> MSELFGVLKSNAGRIILKDPSATSKDVKAYIDSVINTCKNGSITKKAELDEITVDGLDANQVWWQVKLVLDSIDGDLIQGIQELKDVVTPSHNLSDGSTLNSSSGEESELEEAESVFKEKQMLSADVSEIEEQSNDSLSENDEEPSMDDEKTSAEAAREEFAEEKRISSGQDERHSSPDPYGINDKFFDLEKFNRDTLAAEDSNEASEGSEDEDIDYFQDMPSDDEEEEAIYYEDFFDKPTKEPVKKHSDVKDPKEDEELDEEEHDSAMDKVKLDLFADEEDEPNAEGVGEASDKNLSSFEKQQIEIRKQIEQLENEAVAEKKWSLKGEVKAKDRPEDALLTEELEFDRTAKPVPVITSEVTESLEDMIRRRIQDSNFDDLQRRTLLDITRKSQRPQFELSDVKSSKSLAEIYEDDYTRAEDESALSEELQKAHSEISELYANLVYKLDVLSSVHFVPKPASTSLEIRVETPTISMEDAQPLYMSNASSLAPQEIYNVGKAEKDGEIRLKNGVAMSKEELTREDKNRLRRALKRKRSKANLPNVNK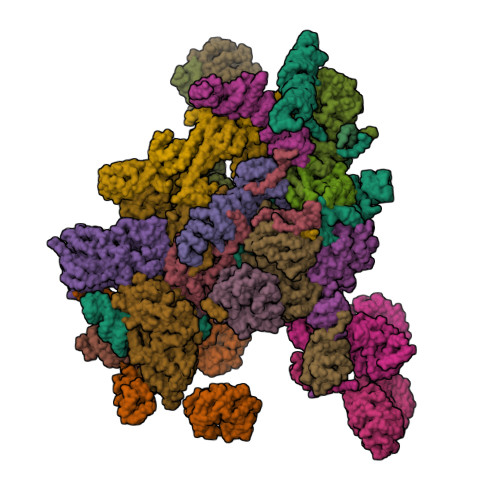RSKRNDVVDTLSKAKNITVINQKGEKKDVSGKTKKSRSGPDSTNIKL;> MSNGHVKFDADESQASASAVTDRQDDVLVISKKDKEVHSSSDEESDDDDAPQEEGLHSGKSEVESQITQREEAIRLEQSQLRSKRRKQNELYAKQKKSVNETEVTDEVIAELPEELLKNIDQKDEGSTQYSSSRHVTFDKLDESDENEEALAKAIKTKKRKTLKNLRKDSVKRGKFRVQLLSTTQDSKTLPPKKESSIIRSKDRWLNRKALNKG;> MTQSLGIEQYKLSVVSGGKPALNNLSSVTGNKNIARLSQDQRNYIIPFNNQIKVYSVETRQCVKTLKFANNSLLSGIFLQEEENNESIVKILLGDITVPQQEDAHLITVFTNNGHVIVLNYKGKLVESPKHFKISLADEKLANVFHSEGNYRILTTFKDPSQKAHNSLQSYRLYALTFDDAKKQFEVAHQAEWHNVILSNISSNGKLLAHMCKDVSTKDHEHKSISVVSLFDDSVNLSFPLGSILSSQTQSLSYNTRYVSSMAIDNMGQQLAVGFASGVISIVSLADLQIRLLKWHIDSVLSLSFSHDGSYLLSGGWEKVMSLWQLETNSQQFLPRLNGIIIDCQVLGPQGNYYSLILQMTENNSNSDYQFLLLNASDLTSKLSINGPLPVFNSTIKHIQQPISAMNTKNSNSITSLNHSKKKQSRKLIKSRRQDFTTNVEINPINKNLYFPHISAVQIFDFYKNEQVNYQYLTSGVNNSMGKVRFELNLQDPIITDLKFTKDGQWMITYEIEYPPNDLLSSKDLTHILKFWTKNDNETNWNLKTKVINPHGISVPITKILPSPRSVNNSQGCLTADNNGGLKFWSFDSHESNWCLKKISLPNFNHFSNSVSLAWSQDGSLIFHGFDDKLQILDFDTFKKFESLENTKTVSEFTLDSEIQTVKLINDTNLIVATRTTLNAINLLRGQVINSFDLYPFVNGVYKNGHMDRLITCDERTGNIALVINQQLTDLDGVPTINYKSRIIIFDSDLSTKLGNFTHHEYISWIGWNYDTDFIFLDIESTLGVVGTXXXXXXXXXXXXXXNDEDEEDIALEFINGEKKDKLVNMNSFTSMFDNIQNVQMDTFFDRVMKVLT;> MSTARPRIITSKAPLLPQQTTPEQRYWRQYTSAQLVKEHNSVTHISFNPQHPHDFAVTSSTRVQIFSSRTRQVIKTFSRFKDVVYSASFRSDGKLLCAGDATGLVSVYDSYNPRTILLSINASTHPTHVTKFHTQDNKILATASDDRVTRLWDISNAYEPQLELTGATDYVRTLSFIPAAPHLVATGSYDGLIRLYDTRSSGSTPIYSLNHDQPVENVIAVSPTQIVSCGGNNFKVWDLTSNKKLYERGNFNKAVTCLDYVENFDSPMQSALIASSLDGHVKVFDPLDNFQVKFGWKFSGPVLSCAVSPSTAQGNRHLVAGLSSGLLAIRTKKKEKRSSDKENAPASFNKNAKSNNFQRMMRGSEYQGDQEHIIHNDKVRSQRRMRAFERNINQFKWSEALDNAFVPGMAKELTLTVLQELRKRGKVRVALYGRDESTLEPLLNWCLKGIEDVRSASIVADWVAVVLELYGNTLESSPVLQELMIDLKTKVRHEIHKSKEAQRIEGMLQLLTS;> XXXXXXXXXXXXXXXXXXXXXXXXXXXXXXXXXXXDHLSKIFLTISKSITQNPWNEENLLPLWLKWLLTLKSGELNSIKDKHTKKNCKHLKSALRSSEEILPVLLGIQGRLEMLRRQAKLREDLAQLSMQEGEDDEIEVIEHSNVISNPLQDQASPVEKLEPDSIVYANGESDEFVDASEYKD;> MDSPVLQSAYDPSGQYLCYVTVALDKQRVGVQPTQRATSSGVDTVWNENFLYLEDSKLKVTCLKWVNLASSDTVAIILGMNNGEIWLYSVLANEVTYKFTTGNSYEIKDIDLMGNQLWCIDSSDAFYQFDLLQFKLLQHFRINNCVQLNKLTIVPAGDSVAQLLVASHSISLIDIEEKKVVMTFPGHVSPVSTLQVITNEFFISGAEGDRFLNVYDIHSGMTKCVLVAESDIKELSHSGQADSIAVTTEDGSLEIFVDPLVSSSTKKRGNKSKKSSKKIQIVSKDGRKVPIYNAFINKDLLNVSWLQNATMPYFKNLQWREIPNEYTVEISLNWNNKNKSADRDLHGKDLASATNYVEGNARVTSGDNFKHVDDAIKSWERELTSLEQEQAKPPQANELLTETFGDKLESSTVARISGKKTNLKGSNLKTATTTGTVTVILSQALQSNDHSLLETVLNNRDERVIRDTIFRLKPALAVILLERLAERIARQTHRQGPLNVWVKWCLIIHGGYLVSIPNLMSTLSSLHSTLKRRSDLLPRLLALDARLDCTINKFKTLNYEAGDIHSSEPVVEEDEDDVEYNEELDDAGLIEDGEESYGSEEEEEGDSDNEEEQKHTSSKQDGRLETEQSDGEEEAGYSDVEME;> MSSLSDQLAQVASNNATVALDRKRRQKLHSASLIYNSKTAATQDYDFIFENASKALEELSQIEPKFAIFSRTLFSESSISLDRNVQTKEEIKDLDNAINAYLLLASSKWYLAPTLHATEWLVRRFQIHVKNTEMLLLSTLNYYQTPVFKRILSIIKLPPLFNCLSNFVRSEKPPTALTMIKLFNDMDFLKLYTSYLDQCIKHNATYTNQLLFTTCCFINVVAFNSNNDEKLNQLVPILLEISAKLLASKSKDCQIAAHTILVVFATALPLKKTIILAAMETILSNLDAKEAKHSALLTICKLFQTLKGQGNVDQLPSKIFKLFDSKFDTVSILTFLDKEDKPVCDKFITSYTRSIARYDRSKLNIILSLLKKIRLERYEVRLIITDLIYLSEILEDKSQLVELFEYFISINEDLVLKCLKSLGLTGELFEIRLTTSLFTNADVNTDIVKQLSDPVETTKKDTASFQTFLDKHSELINTTNVSMLTETGERYKKVLSLFTEAIGKGYKASSFLTSFFTTLESRITFLLRVTISPAAPTALKLISLNNIAKYINSIEKEVNIFTLVPCLICALRDASIKVRTGVKKILSLIAKRPSTKHYFLSDKLYGENVTIPMLNPKDSEAWLSGFLNEYVTENYDISRILTPKRNEKVFLMFWANQALLIPSPYAKTVLLDNLNKSPTYASSYSSLFEEFISHYLENRSSWEKSCIANKTNFEHFERSLVNLVSPKEKQSFMIDFVLSALNSDYEQLANIAAERLISIFASLNNAQKLKIVQNIVDSSSNVESSYDTVGVLQSLPLDSDIFVSILNQNSISNEMDQTDFSKRRRRRSSTSKNAFLKEEVSQLAELHLRKLTIILEALDKVRNVGSEKLLFTLLSLLSDLETLDQDGGLPVLYAQETLISCTLNTITYLKEHGCTELTNVRADILVSAIRNSASPQVQNKLLLVIGSLATLSSEVILHSVMPIFTFMGAHSIRQDDEFTTKVVERTILTVVPALIKNSKGNEKEEMEFLLLSFTTALQHVPRHRRVKLFSTLIKTLDPVKALGSFLFLIAQQYSSALVNFKIGEARILIEFIKALLVDLHVNEELSGLNDLLDIIKLLTSSKSSSEKKKSLESRVLFSNGVLNFSESEFLTFMNNTFEFINKITEETDQDYYDVRRNLRLKVYSVLLDETSDKKLIRNIREEFGTLLEGVLFFINSVELTFSCITSQENEEASDSETSLSDHTTEIKEILFKVLGNVLQILPVDEFVNAVLPLLSTSTNEDIRYHLTLVIGSKFELEGSEAIPIVNNVMKVLLDRMPLESKSVVISQVILNTMTALVSKYGKKLEGSILTQALTLATEKVSSDMTEVKISSLALITNCVQVLGVKSIAFYPKIVPPSIKLFDASLADSSNPLKEQLQVAILLLFAGLIKRIPSFLMSNILDVLHVIYFSREVDSSIRLSVISLIIENIDLKEVLKVLFRIWSTEIATSNDTVAVSLFLSTLESTVENIDKKSATSQSPIFFKLLLSLFEFRSISSFDNNTISRIEASVHEISNSYVLKMNDKVFRPLFVILVRWAFDGEGVTNAGITETERLLAFFKFFNKLQENLRGIITSYFTYLLEPVDMLLKRFISKDMENVNLRRLVINSLTSSLKFDRDEYWKSTSRFELISVSLVNQLSNIENSIGKYLVKAIGALASNNSGVDEHNQILNKLIVEHMKASCSSNEKLWAIRAMKLIYSKIGESWLVLLPQLVPVIAELLEDDDEEIEREVRTGLVKVVENVLGEPFDRYLD;> MSSSLLSVLKEKSRSLKIRNKPVKMTSQERMIVHRCRFVDFTPATITSLAFSHKSNINKLTPSDLRLAIGRSNGNIEIWNPRNNWFQEMVIEGGKDRSIEGLCWSNVNGESLRLFSIGGSTVVTEWDLATGLPLRNYDCNSGVIWSISINDSQDKLSVGCDNGTVVLIDISGGPGVLEHDTILMRQEARVLTLAWKKDDFVIGGCSDGRIRIWSAQKNDENMGRLLHTMKVDKAKKESTLVWSVIYLPRTDQIASGDSTGSIKFWDFQFATLNQSFKAHDADVLCLTTDTDNNYVFSAGVDRKIFQFSQNTNKSQKNNRWVNSSNRLLHGNDIRAICAYQSKGADFLVSGGVEKTLVINSLTSFSNGNYRKMPTVEPYSKNVLVNKEQRLVVSWSESTVKIWTMGTDSSTEQNYKLVCKLTLKDDQNISTCSLSPDGQVLVVGRPSTTKVFHLQPVGNKLKVTKLDNDLLLRTSTKLVKFIDNSKIVICSCEDDVFIVDLESEEDEKPQEVELLEVTSTKSSIKVPYINRINHLEVDQNIAVISRGCGVVDILDLKARISKPLARLNNFITAVHINTSRKSVVVITADNKIYEFNMNLNSEAENEDSESVLTQWSKNNTDNLPKEWKTLKENCVGIFSDIENSSRLWFWGATWISRIDFDVDFPINKXXXXXXXXXXXXXXHFFFTDKYKPLLFVDLISSNELAIIERNPLTFHSKQKAFIQPKLVF;> MKSDFKFSNLLGTVYRQGNITFSDDGKQLLSPVGNRVSVFDLINNKSFTFEYEHRKNIAAIDLNKQGTLLISIDEDGRAILVNFKARNVLHHFNFKEKCSAVKFSPDGRLFALASGRFLQIWKTPDVNKDRQFAPFVRHRVHAGHFQDITSLTWSQDSRFILTTSKDLSAKIWSVDSEEKNLAATTFNGHRDYVMGAFFSHDQEKIYTVSKDGAVFVWEFTKRPSDDDDNESEDDDKQEEVDISKYSWRITKKHFFYANQAKVKCVTFHPATRLLAVGFTSGEFRLYDLPDFTLIQQLSMGQNPVNTVSVNQTGEWLAFGSSKLGQLLVYEWQSESYILKQQGHFDSTNSLAYSPDGSRVVTASEDGKIKVWDITSGFCLATFEEHTSSVTAVQFAKRGQVMFSSSLDGTVRAWDLIRYRNFRTFTGTERIQFNCLAVDPSGEVVCAGSLDNFDIHVWSVQTGQLLDALSGHEGPVSCLSFSQENSVLASASWDKTIRIWSIFGRSQQVEPIEVYSDVLALSMRPDGKEVAVSTLKGQISIFNIEDAKQVGNIDCRKDIISGRFNQDRFTAKNSERSKFFTTIHYSFDGMAIVAGGNNNSICLYDVPNEVLLKRFIVSRNMALNGTLEFLNSKKMTEAGSLDLIDDAGENSDLEDRIDNSLPGSQRGGDLSTRKMRPEVRVTSVQFSPTANAFAAASTEGLLIYSTNDTILFDPFDLDVDVTPHSTVEALREKQFLNALVMAFRLNEEYLINKVYEAIPIKEIPLVASNIPAIYLPRILKFIGDFAIESQHIEFNLIWIKALLSASGGYINEHKYLFSTAMRSIQRFIVRVAKEVVNTTTDNKYTYRFLVSTDGSMEDGAADDDEVLLKDDADEDNEENEENDVVMESDDEEGWIGFNGKDNKLPLSNENDSSDEEENEKELP;> MVKSYQRFEQAAAFGVIASNANCVWIPASSGNSNGSGPGQLITSALEDVNIWDIKTGDLVSKLSDGLPPGASDARGAKPAECTYLEAHKDTDLLAVGYADGVIKVWDLMSKTVLLNFNGHKAAITLLQFDGTGTRLISGSKDSNIIVWDLVGEVGLYKLRSHKDSITGFWCQGEDWLISTSKDGMIKLWDLKTHQCIETHIAHTGECWGLAVKDDLLITTGTDSQVKIWKLDIENDKMGGKLTEMGIFEKQSKQRGLKIEFITNSSDKTSFFYIQNADKTIETFRIRKEEEIARGLKKREKRLKEXXXXXXXXXXYSSFILHPFQTIRSLYKIKSASWTTVSSSKLELVLTTSSNTIEYYSIPYEKRDPTSPAPLKTHTIELQGQRTDVRSIDISDDNKLLATASNGSLKIWNIKTHKCIRTFECGYALTCKFLPGGLLVILGTRNGELQLFDLASSSLLDTIEDAHDAAIWSLDLTSDGKRLVTGSADKTVKFWDFKVENSLVPGTKNKFLPVLKLHHDTTLELTDDILCVRVSPDDRYLAISLLDNTVKVFFLDSMKFYLSLYGHKLPVLSIDISFDSKMIITSSADKNIKIWGLDFGDCHKSLFAHQDSIMNVKFLPQSHNFFSCSKDAVVKYWDGEKFECIQKLYAHQSEVWALAVATDGGFVVSSSHDHSIRIWEETEDXXXXXXXXXXXXXXXXXXXXXXXXXSGVHKQTLESLKAGERLMEALDLGIAEIEGLEAYNRDMKLWQRKKLGEAPIKPQGNAVLIAVNKTPEQYIMDTLLRIRMSQLEDALMVMPFSYVLKFLKFIDTVMQNKTLLHSHLPLICKNLFFIIKFNHKELVSQKNEELKLQINRVKTELRSALKSTEDDLGFNVQGLKFVKQQWNLRHNYEFVDEYDQQEKESNSARKRVFGTVI;> MTMATTAMNVSVPPPDEEEQLLAKFVFGDTTDLQENLAKFNADFIFNEQEMDVEDQEDEGSESDNSEEDEAQNGELDHVNNDQLFFVDDGGNEDSQDKNEDTMDVDDEDDSSSDDYSEDSEEAAWIDSDDEKIKVPILVTNKTKKLRTSYNESKINGVHYINRLRSQFEKIYPRPKWVDDESDSELDDEEDDEEEGSNNVINGDINALTKILSTTYNYKDTLSNSKLLPPKKLDIVRLKDANASHPSHSAIQSLSFHPSKPLLLTGGYDKTLRIYHIDGKTNHLVTSLHLVGSPIQTCTFYTSLSNQNQQNIFTAGRRRYMHSWDLSLENLTHSQTAKIEKFSRLYGHESTQRSFENFKVAHLQNSQTNSVHGIVLLQGNNGWINILHSTSGLWLMGCKIEGVITDFCIDYQPISRGKFRTILIAVNAYGEVWEFDLNKNGHVIRRWKDQGGVGITKIQVGGGTTTTCPALQISKIKQNRWLAVGSESGFVNLYDRNNAMTSSTPTPVAALDQLTTTISNLQFSPDGQILCMASRAVKDALRLVHLPSCSVFSNWPTSGTPLGKVTSVAFSPSGGLLAVGNEQGKVRLWKLNHY;> MSIDLKKRKVEEDVRSRGKNSKIFSPFRIIGNVSNGVPFATGTLGSTFYIVTCVGKTFQIYDANTLHLLFVSEKETPSSIVALSAHFHYVYAAYENKVGIYKRGIEEHLLELETDANVEHLCIFGDYLCASTDDNSIFIYKKSDPQDKYPSEFYTKLTVTEIQGGEIVSLQHLATYLNKLTVVTKSNVLLFNVRTGKLVFTSNEFPDQITTAEPAPVLDIIALGTVTGEVIMFNMRKGKRIRTIKIPQSRISSLSFRTDGSSHLSVGTSSGDLIFYDLDRRSRIHVLKNIHRESYGGVTQATFLNGQPIIVTSGGDNSLKEYVFDPSLSQGSGDVVVQPPRYLRSRGGHSQPPSYIAFADSQSHFMLSASKDRSLWSFSLRKDAQSQEMSQRLHKKQDGGRVGGSTIKSKFPEIVALAIENARIGEWENIITAHKDEKFARTWDMRNKRVGRWTFDTTDDGFVKSVAMSQCGNFGFIGSSNGSITIYNMQSGILRKKYKLHKRAVTGISLDGMNRKMVSCGLDGIVGFYDFNKSTLLGKLKLDAPITAMVYHRSSDLFALALDDLSIVVIDAVTQRVVRQLWGHSNRITAFDFSPEGRWIVSASLDSTIRTWDLPTGGCIDGIIVDNVATNVKFSPNGDLLATTHVTGNGICIWTNRAQFKTVSTRTIDESEFARMALPSTSVRGNDSMLSGALESNGGEDLNDIDFNTYTSLEQIDKELLTLSIGPRSKMNTLLHLDVIRKRSKPKEAPKKSEKLPFFLQLSGEKVGDEASVREGIAHETPEEIHRRDQEAQKKLDAEEQMNKFKVTGRLGFESHFTKQLREGSQSKDYSSLLATLINFSPAAVDLEIRSLNSFEPFDEIVWFIDALTQGLKSNKNFELYETFMSLLFKAHGDVIHANNKNQDIASALQNWEDVHKKEDRLDDLVKFCMGVAAFVTTA;> MKIKTIKRSADDYVPVKSTQESQMPRNLNPELHPFERAREYTKALNATKLERMFAKPFVGQLGYGHRDGVYAIAKNYGSLNKLATGSADGVIKYWNMSTREEFVSFKAHYGLVTGLCVTQPRFHDKKPDLKSQNFMLSCSDDKTVKLWSINVDDYSNKNSSDNDSVTNEEGLIRTFDGESAFQGIDSHRENSTFATGGAKIHLWDVNRLKPVSDLSWGADNITSLKFNQNETDILASTGSDNSIVLYDLRTNSPTQKIVQTMRTNAICWNPMEAFNFVTANEDHNAYYYDMRNLSRSLNVFKDHVSAVMDVDFSPTGDEIVTGSYDKSIRIYKTNHGHSREIYHTKRMQHVFQVKYSMDSKYIISGSDDGNVRLWRSKAWERSNVKTTREKNKLEYDEKLKERFRHMPEIKRISRHRHVPQVIKKAQEIKNIELSSIKRREANERRTRKDMPYISERKKQIVGTVHKYEDSGRDRKRRKEDDKRDTQEK;> MGHKKNGHRRQIKERENQNKFERSTYTNNAKNNHTQTKDKKLRAGLKKIDEQYKKAVSSAAATDYLLPESNGYLEPENELEKTFKVQQSEIKSSVDVSTANKALDLSLKEFGPYHIKYAKNGTHLLITGRKGHVASMDWRKGQLRAELFLNETCHSATYLQNEQYFAVAQKKYTFIYDHEGTELHRLKQHIEARHLDFLPYHYLLVTAGETGWLKYHDVSTGQLVSELRTKAGPTMAMAQNPWNAVMHLGHSNGTVSLWSPSMPEPLVKLLSARGPVNSIAIDRSGYYMATTGADRSMKIWDIRNFKQLHSVESLPTPGTNVSISDTGLLALSRGPHVTLWKDALKLSGDSKPCFGSMGGNPHRNTPYMSHLFAGNKVENLGFVPFEDLLGVGHQTGITNLIVPGAGEANYDALELNPFETKKQRQEQEVRTLLNKLPADTITLDPNSIGSVDKRSSTIRLNAKDLAQTTMDANNKAKTNSDIPDVKPDVKGKNSGLRSFLRKKTQNVIDERKLRVQKQLDKEKNIRKRNHQIKQGLISEDHKDVIEEALSRFG;> MVRKLKHHEQKLLKKVDFLEWKQDQGHRDTQVMRTYHIQNREDYHKYNRICGDIRRLANKLSLLPPTDPFRRKHEQLLLDKLYAMGVLTTKSKISDLENKVTVSAICRRRLPVIMHRLKMAETIQDAVKFIEQGHVRVGPNLINDPAYLVTRNMEDYVTWVDNSKIKKTLLRYRNQIDDFDFS;> MAPIEYLLFEEPTGYAVFKVKLQQDDIGSRLKEVQEQINDFGAFTKLIELVSFAPFKGAAEALENANDISEGLVSESLKAILDLNLPKASSKKKNITLAISDKNLGPSIKEEFPYVDCISNELAQDLIRGVRLHGEKLFKGLQSGDLERAQLGLGHAYSRAKVKFSVQKNDNHIIQAIALLDQLDKDINTFAMRVKEWYGWHFPELAKLVPDNYTFAKLVLFIKDKAXXXXXXXXXXXXXXXXXXXXXXXXXXSETDMENVCVFAQRVASLADYRRQLYDYLCEKMHTVAPNLSELIGEVIGARLISHAGSLTNLSKQAASTVQILGAEKALFRALKTKGNTPKYGLIYHSGFISKASAKNKGRISRYLANKCSMASRIDNYSEEPSNVFGSVLKKQVEQRLEFYNTGKPTLKNELAIQEAMELYNKDKPAAEVEETKEKESSKKRKLEDDDEEKKEKKEKKSKKEKKEKKEKKDKKEKKDKKEKKDKKKKSKD;>[2x]MSFRPGSRGGSRGGSRGGFGGRGGSRGGARGGSRGGFGGRGGSRGGARGGSRGGFGGRGGSRGGARGGSRGGRGGAAGGARGGAKVVIEPHRHAGVYIARGKEDLLVTKNMAPGESVYGEKRISVEEPSKEDGVPPTKVEYRVWNPFRSKLAAGIMGGLDELFIAPGKKVLYLGAASGTSVSHVSDVVGPEGVVYAVEFSHRPGRELISMAKKRPNIIPIIEDARHPQKYRMLIGMVDCVFADVAQPDQARIIALNSHMFLKDQGGVVISIKANCIDSTVDAETVFAREVQKLREERIKPLEQLTLEPYERDHCIVVGRYMRSGLKK;>[2x]MSAPNPKAFPLADAALTQQILDVVQQAANLRQLKKGANEATKTLNRGISEFIIMAADCEPIEILLHLPLLCEDKNVPYVFVPSRVALGRACGVSRPVIAASITTNDASAIKTQIYAVKDKIETLLI;> MSDVTQQKKRKRSKGEVNPSKPTVDEEITDPSSNEDEQLEVSDEEDALESEEEFEGENPADKRRRLAKQYLENLKSEANDILTDNRNAEEKDLNNLKERTIDEYNNFDAGDLDKDIIASRLKEDVAEQQGRVFRYFGDKLLISEAKQSFTRVGENNLTCISCFQPVLNKYTFEESSNGDKNKGRLFAYTVSKDLQLTKYDITDFSKRPKKLKYAKGGAKYIPTSKHEYENTTEGHYDEILTVAASPDGKYVVTGGRDRKLIVWSTESLSPVKVIPTKDRRGEVLSLAFRKNSDQLYASCADFKIRTYSINQFSQLEILYGHHDIVEDISALAMERCVTVGARDRTAMLWKIPDETRLTFRGGDEPQKLLRRWMKENAKEGEDGEVKYPDESEAPLFFCEGSIDVVSMVDDFHFITGSDNGNICLWSLAKKKPIFTERIAHGILPEPSFNDISGETDEELRKRQLQGKKLLQPFWITSLYAIPYSNVFISGSWSGSLKVWKISDNLRSFELLGELSGAKGVVTKIQVVESGKHGKEKFRILASIAKEHRLGRWIANVSGARNGIYSAVIDQTGF;> MGKAKKTRKFGLVKRTLNTKKDQRLKKNQENIKTKEDPELTRNIPQVSSALFFQYNQAIKPPYQVLIDTNFINFSIQKKVDIVRGMMDCLLAKCNPLITDCVMAELEKLGPKYRIALKLARDPRIKRLSCSHKGTYADDCLVHRVLQHKCYIVATNDAGLKQRIRKIPGIPLMSVGGHAYVIEKLPDVF>EKQTAKRNRREEILQSLALMLESSDGSQRITTAKLAASVGVSEAALYRHFPSKTRMFDSLIEFIEDSLITRINLILKDEKDTTARLRLIVLLI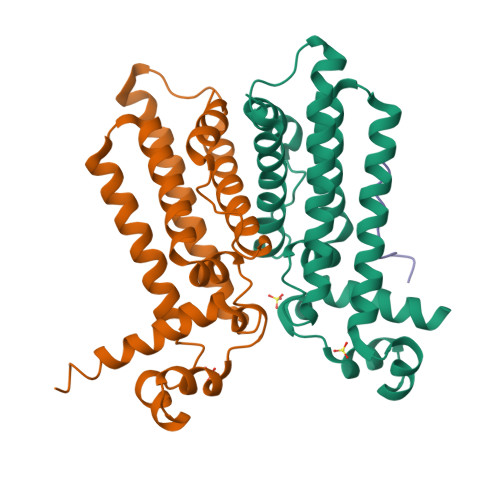LGFGERNPGLTRILTGHALMFEQDRLQGRINQLFERIEAQLRQVMREKKMREGEGYTLDETLLASQLLAFCEGMLSRFVRSEFKYRPTDDFDARWPLVAAQLQ[2x];> LDIPAFLRKQA> ATQQEICKNMWDPFQSMRAVTGLMELTSGQCTQLSKDAAAILAGVKESHDSISVDKNYKVL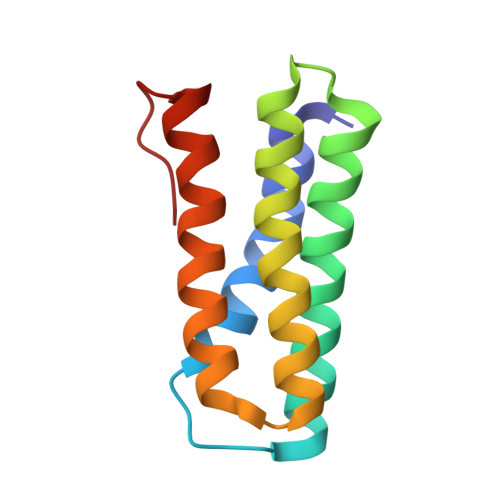NDEVAYHAANIDAAAKANDLEEVQVQFRRMTIACRNCHKIYKTEQRLVP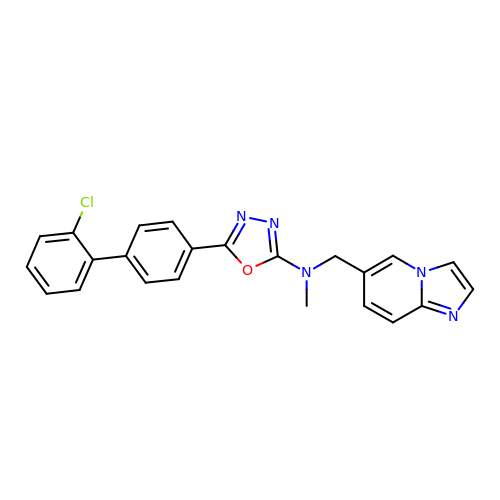5-(2'-chloro-[1,1'-biphenyl]-4-yl)-N-(imidazo[1,2-a]pyridin-6-ylmethyl)-N-methyl-1,3,4-oxadiazol-2-amine | C23 H18 Cl N5 O | WPRJOLMYEVNSEK-UHFFFAOYSA-N> DPSTYADYFSAWDKWEKQALPGEERDEAVSRLKECLINNSDELR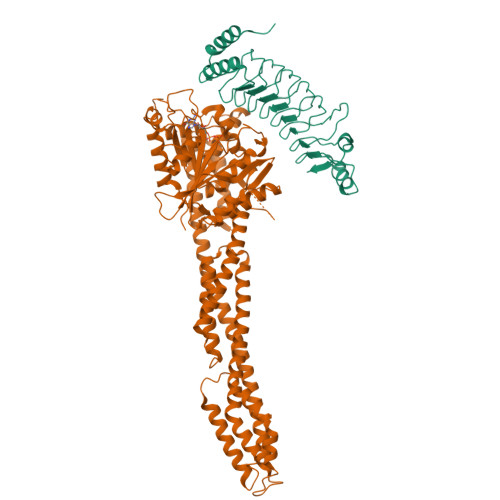LDRLNLSSLPDNLPAQITLLNVSYNQLTNLPELPVTLKKLYSASNKLSELPVLPPALESLQVQHNELENLPALPDSLLTMNISYNEIVSLPSLPQALKNLRATRNFLTELPAFSEGNNPVVREYFFDRNQISHIPESILNLRNECSIHISDNPLSSHALQALQRLTSSPDYHGPRIYFSMSD;> MDPMASEIHMTGPMCLIENTNGRLMANPEALKILSAITQPMVVVAIVGLYRTGKSYLMNKLAGKKKGFSLGSTVQSHTKGIWMWCVPHPKKPGHILVLLDTEGLGDVEKGDNQNDSWIFALAVLLSSTFVYNSIGTINQQAMDQLYYVTELTHRIRSKSSPDENENEVEDSADFVSFFPDFVWTLRDFSLDLEADGQPLTPDEYLTYSLKLKKGTSQKDETFNLPRLCIRKFFPKKKCFVFDRPVHRRKLAQLEKLQDEELDPEFVQQVADFCSYIFSNSKTKTLSGGIQVNGPRLESLVLTYVNAISSGDLPCMENAVLALAQIENSAAVQKAIAHYEQQMGQKVQLPTETLQELLDLHRDSEREAIEVFIRSSFKDVDHLFQKELAAQLEKKRDDFCKQNQEASSDRCSALLQVIFSPLEEEVKAGIYSKPGGYRLFVQKLQDLKKKYYEEPRKGIQAEEILQTYLKSKESMTDAILQTDQTLTEKEKEIEVERVKAESAQASAKMLHEMQRKNEQMMEQKERSYQEHLKQLTEKMENDRVQLLKEQERTLALKLQEQEQLLKEGFQKESRIMKNEIQDLQTKMRRRKACTIS>SILTFEERDTSSLSIEARLESIEEKLSMILGLLRTLNIATAGPTAARDGIRDAMIGVREELIADIIKEAKGKAAEMMEEE[8x]

For all paramyxoviruses, the nucleoprotein (N) encapsidates viral RNA, leading to a N-RNA complex which, together with the RNA-dependent RNA polymerase (L) and the phosphoprotein (P), forms the viral replication complex. The P protein is thought to be responsible for the recruitment of the large polymerase L onto the viral N-RNA template through direct interactions with N and L. In addition, P chaperones the nascent N, which is sequestered in the form of an RNA-free NP complex. For all members of the Paramyxoviridae family, the P protein is an intrinsically disordered polypeptide which forms tetramers through a central α-helical coiled-coil region. The analysis predicts the presence of a central, highly conserved region with α-helical propensity located between residues 158 to 237, which we refer to as Pced.

A single diffracting crystal of HMPV Pced grew after 140 days, suggesting degradation occurred in the drop prior to crystallization. Diffraction data were phased by molecular replacement using residues 169 to 194 from Pcore, revealing a tetrameric α-helical arrangement consistent with the modeled structure. The asymmetric unit contains 2 tetramers, with a solvent content of 40%. Since the asymmetric unit could not physically contain 2 tetramers with residues 158-237 (with 1 tetramer present the solvent content is 16%), packing considerations suggest that degradation necessarily occurred prior to crystallization. The residues 158-168 and 195-237 are absent from the structure, in line with the flexibility observed for these regions by MDS and SAXS-based ensemble optimization. Additional stability is provided by a solvent-exposed network of ionic interactions created by Glu173/Glu177 and Arg175, or Glu180 and Lys182 side chains from neighbouring protomers. Comparison with representative models from the SAXS optimized ensembles, as well as with the best scoring models from MDS demonstrates Cα RMSDs ranging from 0.9 to 1.6 Å over aligned residues, confirming the accuracy of the modeled Pcore. The structural data presented here indicates that the α-helical tetramerization domain of HMPV P (residues 171-194) is considerably shorter than the highly conserved central region of the molecule (residues 158-237). Interestingly, the sequence of Pcore aligns with a region of RSV P that is necessary for coimmunoprecipitation of the L protein, suggesting either direct binding to L or the requirement of a tetrameric P protein for efficient P-L association. The short tetrameric coiled coil from HMPV P clusters in a separate branch from SeV/MuV/MeV and RV/VSV, emphasizing the pertinence of its classification as a separate subfamily, Pneumovirinae.> AMKKDSKAP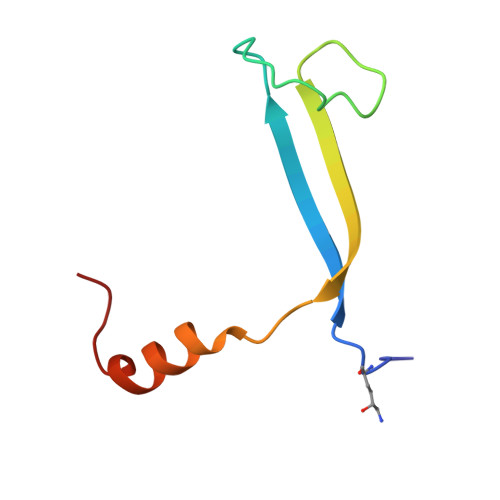CVEVFDERDGCKAAGTQKASGDDGFCVKVSMKAIKMNAAEATSVTKNYNTKLL1-(3-PHENYL-1H-PYRAZOL-5-YL)CYCLOPENTANOL 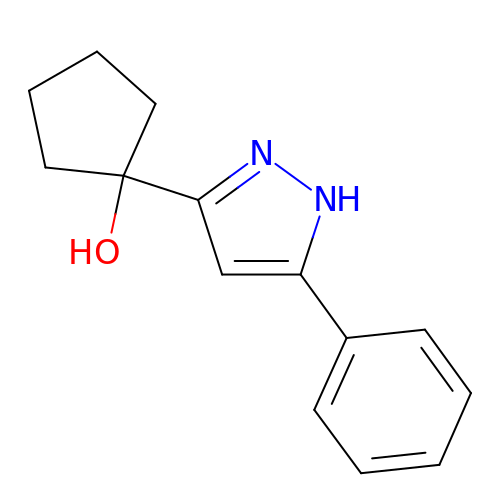| C14 H16 N2 O | GKHXBOMLCZWNOE-UHFFFAOYSA-N> SPSAEECGYSDRVRSMTLGNSTITTQESANVVVGYGEWPSYLSDREATAEDQPTQPDVATCRFYTLESVQWEKTSPGWWWKFPEALKNMGLFGQNMHYHYLGRAGYTIHVQCNASKFHQGCLLVVCVPEAEMGCADTDTTFPATELTTEDTPHVFTSDSITGKKVQAAVCNAGMGVGVGNLTIFPHQWINLRTNNSATIVIPYINSVPMDNMFRHYNFTLMIIPFAPLNFTDGATAYV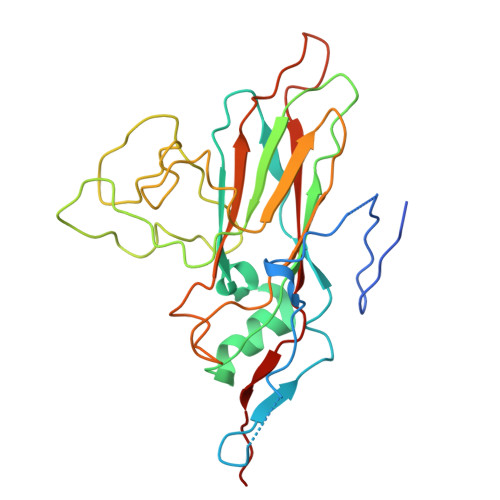PITVTIAPMYAEYNGLRLAST>MNPPTTTTTTTRTIRAPKVQLTPNSATRRRRNRRRRRPAAAIAGPLSIQPSSINRRMVSRVTRRSAVVTAAGLAWLRQYLNPMGPDTTSVTGYPDGSAVTTCIADYSNTFNVSFPPREALYCTGSSSSEKPTLVDADNYAKIDKWSNYDITLCVLALPMLR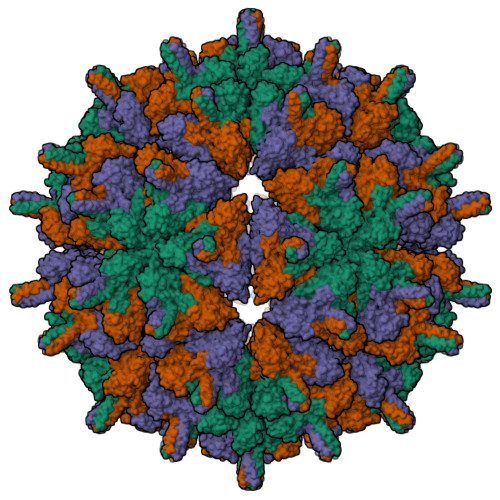NVVMLRLYPHTPTAFALTEQTPNFPQRFPNWSVYSADGTRFNNGDEPGYLQSYVYLPNVDKHLSAARGYRLLSRGITGIFSAPALETQGFVTACQYLAEGSIQSQSIKSDAVRSVTVNSDGTVKNVESSSQTVSSMPRYVFPLDGDNCAPSSLTETYHQAYQSKATDGFYMPVLSSSRDNPFHPPQPRAIAVYGSFLARGCLDPVSEAHEADGPTHDIYRLNVADDVAPLFNTGVVWFEGISPKFSLKLKTRTVLQYIPTSGSVLANFTRHEPTYDQIALDAADRLRNLMPHAYPAAYNDWGWLGDLLDSAISMLPGVGTVYNIAKPLIKPAWNWLGNKVSDFFGNPVARDGDIFFDAK[3x]3-({11-[3-(4-chloro-3,5-dimethylphenoxy)propyl]-1-oxo-7-(1,3,5-trimethyl-1H-pyrazol-4-yl)-4,5-dihydro-1H-[1,4]diazepino[1,2-a]indol-2(3H)-yl}methyl)benzoic 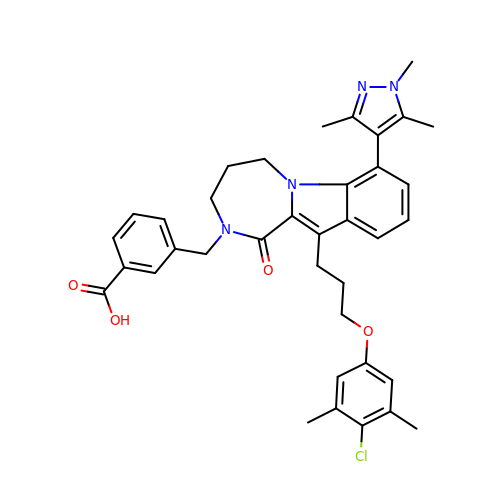acid | C37 H39 Cl N4 O4 | VMBSCFPYXBSHSU-UHFFFAOYSA-N>[7x]MADSDINIKTGTTDIGSNTTVKTGDLVTYDKENGMHKKVFYSFIDDKNHNKKLLVIRTKGTIAGQYRVYSEEGANKSGLAWPSAFKVQLQLPDNEVAQISDYYPRNSIDTKEYMSTLTYGFNSNVTGDDTGKIGGLIGANVSIGHTLRY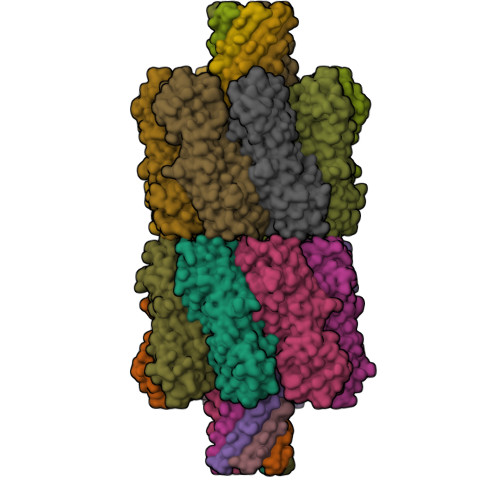VQPDFKTILESPTDKKVGWKVIFNNMVNQNWGPYDRDSWNPVYGNQLFMKTRNGSMKAADNFLDPNKASSLLSSGFSPDFATVITMDRCASKQQTNIDVIYERVRDDYQLHWTSTNWKGTNTKDKWTDRSSERYKIDWEKEEMTNGSSGSVTTLSGLSGEQGPSGDMTTEEDSATHIKFSKRDEDGRELAGATMELRDSSGKTISTWISDGHVKDFYLYPGKYTFVETAAPDGYEVATPIEFTVNEDGQVTVDGEATEGDAHTGGSHHHHHH;>[7x]MADSDINIKTGTTDIGSNTTVKTGDLVTYDKENGMHKKVFYSFIDDKNHNKKLLVIRTKGTIAGQYRVYSEEGANKSGLAWPSAFKVQLQLPDNEVAQISDYYPRNSIDTKEYMSTLTYGFNSNVTGDDTGKIGGLIGANVSIGHTLRYVQPDFKTILESPTDKKVGWKVIFNNMVNQNWGPYDRDSWNPVYGNQLFMKTRNGSMKAADNFLDPNKASSLLSSGFSPDFATVITMDRCASKQQTNIDVIYERVRDDYQLHWTSTNWKGTNTKDKWTDRSSERYKIDWEKEEMTNGSSGSRGVPHIVMVDAYKRYKGGSHHHHHH> AWSHPQFEKTPATQPLINAEPAVAAQTEQNPQVGQVMPGVQGADAPVVAQNGPSRDVKLTFAQIAPPPGSMVLRGINPNGSIEFGMRSDEVVTKAMLNLEYTPSPSLLPVQSQLKVYLNDELMGVLPVTKEQLGKKTLAQMPIN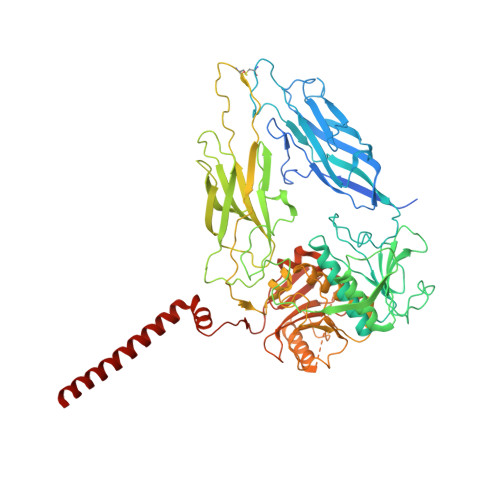PLFISDFNRVRLEFVGHYQDVCEKPASTTLWLDVGRSSGLDLTYQTLNVKNDLSHFPVPFFDPSDNRTNTLPMVFAGAPDVGLQQASAIVASWFGSRSGWRGQNFPVLYNQLPDRNAIVFATNDKRPDFLRDHPAVKAPVIEMINHPQNPYVKLLVVFGRDDKDLLQAAKGIAQGNILFRGESVVVNEVKPLLPRKPYDAPNWVRTDRPVTFGELKTYEEQLQSSGLEPAAINVSLNLPPDLYLMRSTGIDMDINYRYTMPPVKDSSRMDISLNNQFLQSFNLSSKQEANRLLLRIPVLQGLLDGKTDVSIPALKLGATNQLRFDFEYMNPMPGGSVDNCITFQPVQNHVVIGDDSTIDFSKYYHFIPMPDLRAFANAGFPFSRMADLSQTITVMPKAPNEAQMETLLNTVGFIGAQTGFPAINLTVTDDGSTIQGKDADIMIIGGIPDKLKDDKQIDLLVQATESWVKTPMRQTPFPGIVPDESDRAAETRSTLTSSGAMAAVIGFQSPYNDQRSVIALLADSPRGYEMLNDAVNDSGKRATMFGSVAVIRESGINSLRVGDVYYVGHLPWFERVWYALANHPILLAVLAAISVILLAWVLWRLLRIISRRRLNPDNE>[4x]GARDDEYDYLFKVVLIGDSGVGKSNLLSRFTRNEFNLESKSTIGVEFATRSIQVDGKTIKAQIWDTAGLERYRAI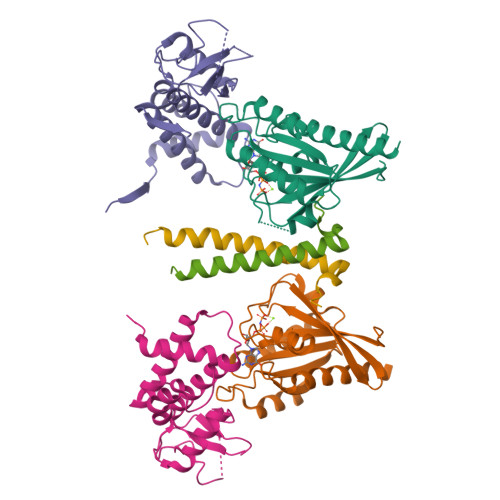TSAYYRGAVGALLVYDIAKHLTYENVERWLKELRDHADSNIVIMLVGNKSDLRHLRAVPTDEARAFAEKNGLSFIETSALDSTNVEAAFQTILTEIYRIVSQKQMSDRRE;>[4x]GAASNKSTSSAMSGSHQDLSVIQPIVKDCKEADLSLYNEFRLWKDEPTMDRTCPFLDKIYQEDIFPCLTFSKSELASAVLEAVENNTLSIEPVGLQPIRFVKASAVECGGPKKCALTGQSKSCKHRIKLGDSSNYYYISPFCRYRITSVCNFFTYIRYIQQGLVKQQDVDQMFWEVMQLRKEMSLAKLGYFKEEL;>GAASGAKSLFSTAFSESLAAEISSVSRDELMEAIQKQEEINFRLQDYIDRIIVAIMETNPSILEVK[4x]> LSYRCPCRFFESHIARANVKHLKILNTPNCA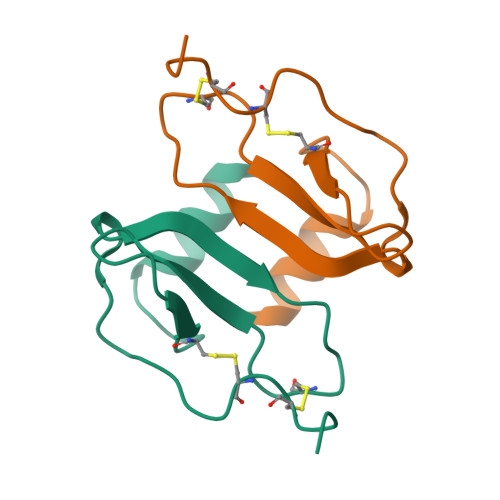LQIVARLKNNNRQVCIDPKLKWIQEYLEKALN>HHHHHHENLYFQSNMSFDNYLVPTVIEQSGRGERAFDIYSRLLKERIVFLVGPVTDESANLVVAQLLFLESENPDKDIFFYINSPGGSVTAGMSIYDTMNFIKPDVSTLCLGQAASMGAFLLSAGEKGKRFALPNSRIMIHQPLISGGLGGQASDIEIHARELLKIKEKLNRLMAKHCDRDLADLERDTDRDNFMSAEEAKEYGLIDQILENRAS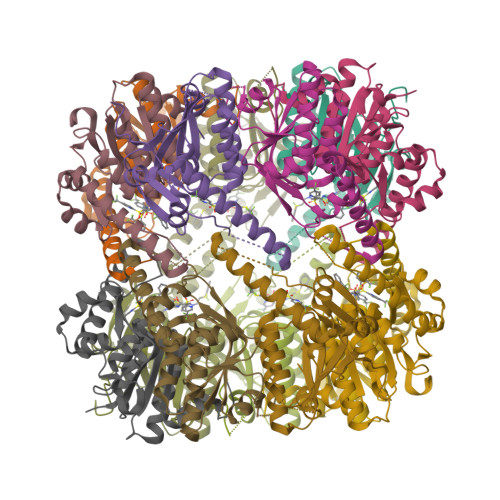LRL[7x]Candida boidinii NAD+-dependent formate dehydrogenase (CbFDH) is a homodimeric 82 kDa enzyme complex that catalyzes the reversible conversion of formate and carbon dioxide using NAD+/NADH coenzymes for electron transfer. Candida boidinii NAD+-dependent formate dehydrogenase (CbFDH) has gained significant attention for its potential application in the production of biofuels and various industrial chemicals from inorganic carbon dioxide. Here, we present high-resolution crystal structures of apo CbFDH determined at cryogenic and ambient temperatures, as well as as that of the highly active Val120Thr mutant of CbFDH at cryogenic temperature. The inherent capability of the enzyme to catalyze the conversion of CO2 to formate holds significant potential for reducing atmospheric CO2 levels.

Studying protein structures at ambient temperature offers valuable insights into their natural conformational dynamics, active-site flexibility, functional mechanisms and binding behavior. Therefore, in addition to the structure obtained at cryogenic temperature, we also determined the structure of wild-type CbFDH at ambient temperature. 97.66% of the residues were in the favored regions, while 2.34% were in the allowed regions, with no outliers according to the Ramachandran statistics. Comparison of the wild-type structures determined at cryogenic and ambient temperatures showed that the structure did not significantly change due to temperature except for flexible loops and large amino-acid side chains. The reason might be that flash-cooling in liquid nitrogen captured the protein in its most stable state in solution, which we also observed in the ambient temperature structure. The cryogenic temperature structure exhibited a significantly higher number of identified water molecules, with 2179 waters resolved, compared with the ambient temperature structure with only 393 water molecules. The higher resolution achieved at cryogenic temperatures significantly improves the accuracy of identifying water molecules compared with the ambient temperature structures at lower resolution. Another reason for the different numbers of identified water molecules could be the differences in water accessibility and occupancy between the two conditions. At cryogenic temperatures water molecules might be frozen at specific binding sites, leading to the stabilization of interactions that are transient at ambient temperature.

>MKIVLVLYDAGKHAADEEKLYGCTENKLGIANWLKDQGHELITTSDKEGGNSVLDQHIPDADIIITTPFHPAYITKERIDKAKKLKLVVVAGVGSDHIDLDYINQTGKKISVLEVTGSNVVSVAEHVLMTMLVLVRNFVPAHEQIINHDWEVAAIAKDAYDIEGKTIATIGAGRIGYRVLERLVPFNPKELLYYDYQALPKDAEEKVGARRVENIEELVAQADIVTINAPLHAGTKGLINKELLSKFKKGAWLVNTARGAICVAEDVAAALESGQLRGYGGDVWFPQPAPKDHPWRDMRNKYGAGNAMTPHYSGTTLDAQTRYAEGTKNILESFFTGKFDYRPQDIILLNGEYITKAYGKHDKK[4x]6-{5-[(2-aminopyrimidin-4-yl)amino]-2-hydroxyphenyl}-N-methylidene-1-benzothiophene-2-carboxamide 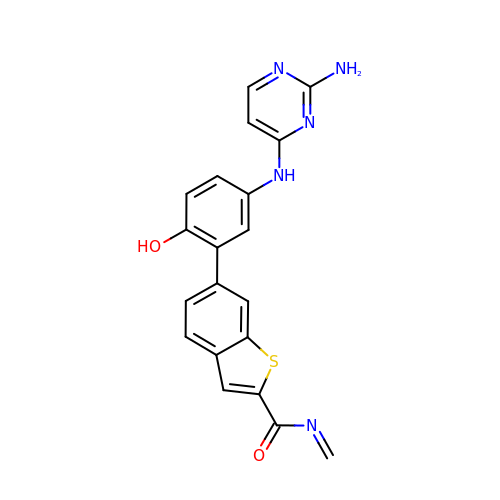| C20 H15 N5 O2 S | KCQAKLMJFBAMFX-UHFFFAOYSA-N>MKVQYSFEREFEELMSDLLSKYGYEMFQMDGLGDQLDVVKFTEDFVRRGIIESTIDANANVRVTNISTYFIEISKPHTYLYSLYRIWQKMKEMFGKGVADEFVEAQINGAVYLHDRHHAALMPYCFAYTLKPIVEKGLPFIKTIKSEPAKHLSTFIQHVIQFVMFASNQSSGAVGLPDFFVWMWYFVKKDLKEGIIPRDKLDWYIEQHFQILTYSLNQPIRTTQSPYTNFTYLDRNYIKAIFEGERYPDGSLITDHVEDIIALQKHYWEWVSRERERQMFTFPVLTASLLYKDGKFLDEDSARFINKINMKWQDTNWYISDSIDAVASCCRLTSSTQTLKKFSLSSEEEEKLKGRMNSIGGSDLNIGSFKVITVNLPRIALESGGDREKYLQILRHRVQLIKKALAAVREIIKERISEGLLPLYENGLMLLNRQYGTIGVTGVW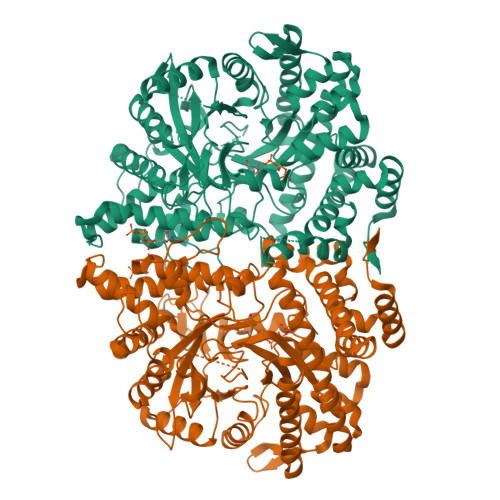ESASIMGLTTEDIDGLKYTEEGEVFVDNVLDTIREEAEKGYHEYGFTFNIEQVPAEKAAVTLAQKDRFLFGEKQPFEIYSNQWVPLMANTDVLNRIRYSGKWDKKVSGGAILHINLGESFKTEEESFNMVKMIADMGVMYFAFNTKISVCEDGHAFYGERCPVCGKAKVDEYMRIVGYLVPVSAFNKERREIEYPRRQFYDSLTIRR[2x]>[4x]MKVLVTGFEPFGGEKINPTERIAKDLDGIKIGDAQVFGRVLPVVFGKAKEVLEKTLEEIKPDIAIHVG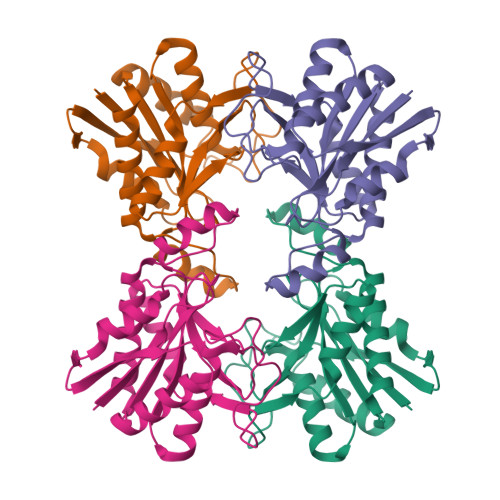LAPGRSAISIERIAVNAIDARIPDNEGKKIEDEPIVPGAPTAYFSTLPIKKIMKKLHERGIPAYISNSAGLYLSNYVMYLSLHHSATKGYPKMSGFIHVPYIPEQIIDKIGKGQVPPSMSYEMQLEAVKVAIEVALEELL> APDTSVSNKQNFST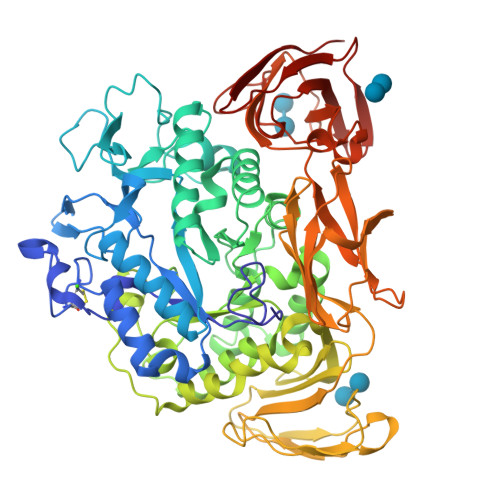DVIYQIFTDRFSDGNPANNPTGAAFDGTCTNLRLYCGGDWQGIINKINDGYLTGMGVTAIWISQPVENIYSIINYSGVNNTAYHGYWARDFKKTNPAYGTIADFQNLIAAAHAKNIKVIIDFAPNHTSPASSDQPSFAENGRLYDNGTLLGGYTNDTQNLFHHNGGTDFSTTENGIYKNLLDLADLNHNNSTVDVYLKDAIKMWLDLGIDGIRMDAVKHMPFGWQKSFMAAVNNYKPVFTFGEWFLGVNEVSPENHKFANESGMSLLDFRFAQKVRQVFRDNTDNMYGLKAMLEGSAADYAQVDDQVTFIDNHDMERFHASNANRRKLEQALAFTLTSRGVPAIYYGTEQYMSGGTDPDNRARIPSFSTSTTAYQVIQKLAPLRKCNPAIAYGSTQERWINNDVLIYERKFGSNVAVVAVNRNLNAPASISGLVTSLPQGSYNDVLGGLLNGNTLSVGSGGAASNFTLAAGGTAVWQYTAATATPTIGHVGPMMAKPGVTITIDGRGFGSSKGTVYFGTTAVSGADITSWEDTQIKVKIPAVAGGNYNIKVANAAGTASNVYDNFEVLSGDQVSVRFVVNNATTALGQNVYLTGSVSELGNWDPAKAIGPMYNQVVYQYPNWYYDVSVPAGKTIEFKFLKKQGSTVTWEGGSNHTFTAPSSGTATINVNWQP>[3x]MAGGRHRRVVGTLHLLLLVAALPWASRGVSPSASAWPEEKNYHQPAILNSSALRQIAEGTSISEMWQNDLQPLLIERYPGSPGSYAARQHIMQRIQRLQADWVLEIDTFLSQTPEGERSFSNIISTLNPTAKRHLVLACHYDSKYFSHWNNRVFVGATDSAVPCAMMLELARALDKKLLSLKTVSDSKPDLSLQLIFFDGEEAFLHWSPQDSLYGSRHLAAKMASTPHPPGARGTSQLHGMDLLVLLDL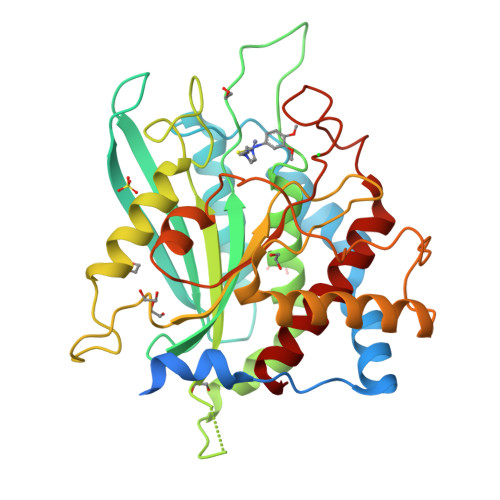IGAPNPTFPNFFPNSARWFERLQAIEHELHELGLLKDHSLEGRYFQNYSYGGVIQDDHIPFLRRGVPVLHLIPSPFPEVWHTMDDNEENLDESTIDNLNKILQVFVLEYLHL>MALPTPSDSTLPAEARGRGR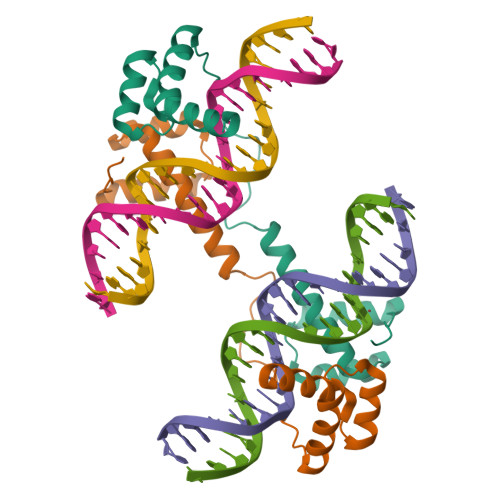RRRLVWTPSQSEALRACFERNPYPGIATRERLAQAIGIPEPRVQIWFQNERSRQLRQHRRESRPWPGRRGPPEGRRKRTAVTGSQTALLLRAFEKDRFPGIAAREELARETGLPESRIQIWFQNRRARHP[2x]> MKPTYEILGQMDETFILVKDSEYLYFVDQHLLEERINYEKLKDENLACRISVKAGQKLSEEKIRELIKTWRNLENPHVCPHGTPIYYKIPLREIYEKVGRNY

MutLs, with a few exceptions, are endonucleases that incise the error-containing (i.e., newly synthesized) strand of the mismatched duplex. Prokaryotic MutL endonucleases and the endonuclease subunits of eukaryotic MutL homologs include two domains: the N-terminal ATPase domain and the C-terminal endonuclease domain (CTD). The dimerization subdomain contains the metal-binding sites, in which multiple zinc ions are coordinated by the residues from highly conserved motifs: DQHAX2EX4E, ACR, and CPHGRP (underlined residues coordinate the zinc ions). Here, we solved the crystal structure of the endonuclease domain of Aquifex aeolicus MutL in the manganese- or cadmium-bound form, revealing that these metals compete with zinc at the same sites.

Arg406 is a component of the CPHGRP motif and completely conserved in all MutL endonucleases including human PMS2 and MLH3, the nuclease subunits of MutLα and MutLγ, respectively. Arg406 of aqMutL corresponds to Arg847 of human PMS2. The R847T mutation has been found in Lynch syndrome-suspicious patients and registered as a variant of uncertain significance at the ClinVar database. The R406T mutant form of the aqMutL CTD was crystallized in the presence of cadmium ion, and the structure was solved with the Cd-SAD phasing. As was expected from the CD measurements, the overall structure was almost identical to that of the WT aqMutL CTD. The distance between the M1 cadmium ion and the W1 water molecule was 2.57 Å. However, the position of the α4 helix, the local structure around Thr406, and the quaternary structure were the same as those of the zinc-bound form of the WT aqMutL CTD (respectively). These results support the notion that the M1 cadmium ion fixes the side chain of Arg406 of aqMutL, causing the shift in the position of the α4 helix and the change in the quaternary structure. The DNA-binding ability of aqMutL was not influenced by these mutations, whereas the endonuclease activity was severely impaired by the R406A and R406T mutations. The R406K mutant form retained significant, albeit weaker, endonuclease activity. These results suggest that the Arg residue in the CPHGRP motif is a catalytic residue for the endonuclease activity.> MDGEGFGELLQQAEQLAAETEGVTELPHVERNLQEIQQAGERLRSKTMTRTSQESANVKASVLLGSRGLDISHISQRLESLSAATTFEPLEPVKDTDIQGFLKNEKDNALLSAIEESRKRTFVMAEEYHRESMLVEWEQVKQRVLHTLLASGEDALDFTQESETSYISESGAPGRSSLDNVEMAYARQMYMYNEKVVSGHLQPSLVDLCTEAAERLDDKNVSDLWVMVKQMTDVPLIPASDTLKSRCSGQMQMAFVRQALNYLEQSYKNYTLISVFANLQQAQLGGVPGTYNLVRSFLNIRLPTPIPGLQDGEIEGYPVWALIYYCMRCGDLMAAQQVVNRAQHQLGDFKNCFQEYIHNKDRRLSPTTENKLRLHYRRAVRASTDPYKRAVYCIIGRCDVSDNHSEVADKTEDYLWLKLSQVCFEDEANSSPQDRLTLPQFQKQLFEDYGESHFAVNQQPYLYFQVLFLTAQFEAAIAFLFRLERTRCHAVHVALALFELKLLLKSTGQSAQLLSQEPGEPQGVRRLNFIRLLMLYTRKFEPTDPREALQYFYFLRNEKDNQGESMFLRCVSELV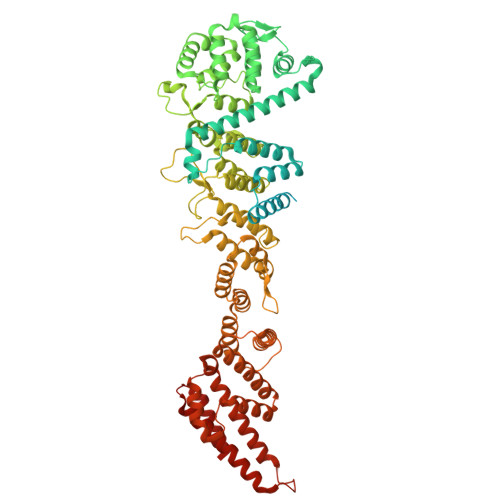IESREFDMLLGKLEKDGSRKPGAIDKFTRDTKTIINKVASVAENKGLFEEAAKLYDLAKNPDKVLELTNKLLSPVVSQISAPQSNRERLKNMALAIAERYKSQGVSAEKSINSTFYLLLDLITFFDEYHAGHIDLSFDVIERLKLVPLSQDSVEERVAAFRNFSDEIRHNLSEILLATMNILFTQYKRLKGSGPTTLGRPQRVQEDKDSVLRSQARALITFAGMIPYRMSGDTNARLVQMEVLMN>SGF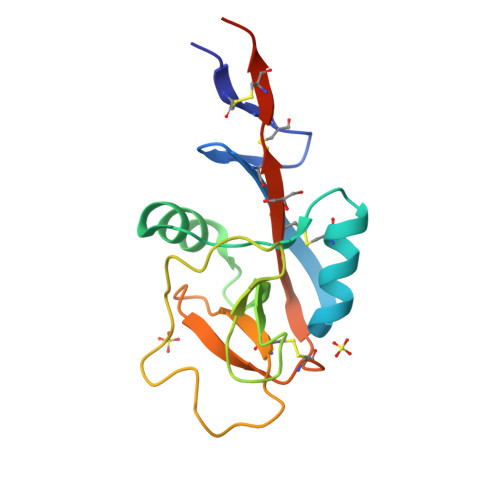VCNTCPEKWINFQRKCYYFGKGTKQWVHARYACDDMEGQLVSIHSPEEQDFLTKHASHTGSWIGLRNLDLKGEFIWVDGSHVDYSNWAPGEPTARSQGEDCVMMRGSGRWNDAFCDRKLGAWVCDRLATCTPPASEGSAE[4x]4-methyl-5-[3-(methylsulfanyl)-1H-pyrazol-5-yl]-2-thiophen-2-yl-1,3-thiazole 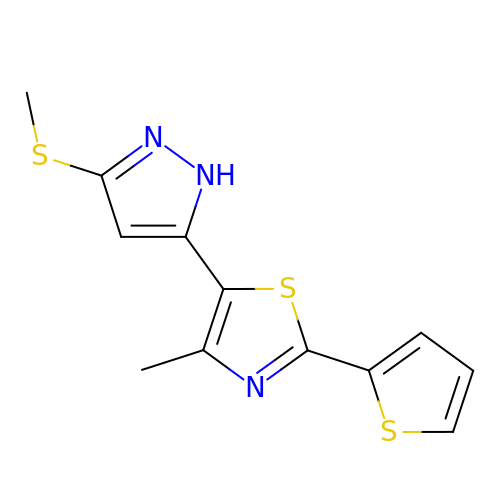| C12 H11 N3 S3 | QVFLVBFBDVWAJG-UHFFFAOYSA-N Prolidases, also known as Xaa-Pro dipeptidases, are metalloproteases that catalyze the hydrolysis of dipeptides containing a C-terminal proline residue. Prolidases share a number of conserved sequence and structural features. These enzymes possess an N-terminal domain and a C-terminal catalytic domain, and form dimers through contact between both domains in a head-to-tail arrangement. The catalytic site features a binuclear metal cluster in the center of a pita-bread fold that is a canonical feature of this family of enzymes. Here we report the structure of E. coli PepQ, showing it to have the predicted pita-bread fold.

To better understand the potential significance of sequence conservation between the E. coli and human prolidases, we solved the structure of the bacterial enzyme at 2.0 Å resolution. The asymmetric unit contains a single PepQ dimer, which is the native oligomeric structure of this protein, arranged head-to-tail with inter-dimer contacts made between both domains. The active site of E. coli PepQ also features canonical metal binding residues, Asp246, Asp257, His339, Glu384 and Glu423, chelating two metal ions. Because PepQ was crystallized in buffer containing magnesium, the density found in this region is most likely derived from magnesium ions. Additionally, the mF0-DFc difference map shows greater density for one of the two metal ions (chelated by His339), consistent with reports from other pita-bread fold peptidases that this binding site has a higher affinity for metal ions. The decreased occupancy at the second metal site is surprising, given that the magnesium concentration during crystallization was in the millimolar range. This observation suggests that the affinity for magnesium of either PepQ in general, or this site in particular, is not as high as seen for the preferred manganese ion in related proteins, reported to be in the low- or sub-micromolar range [22], [34], [41]. Asp45, which reaches into the active site of one monomer from a loop region in the N-terminal domain of the other monomer, is seen in E. coli to be within interaction distance of Arg370, with the charged ends of the side chains approximately 3.5Å apart. PepQ Arg370, which is projected further into the active site on one of the loop regions conserved in prolidases from higher organisms, is placed far enough into the active site that it would physically impede the binding of longer peptides, as seen in the overlap between this arginine and the PepP-bound substrate tripeptide. PepQ R370 is, however, in an appropriate position for the guanidinium group of the arginine to interact with the C-terminus of the proline residue.

>[2x]MESLASLYKNHIATLQERTRDALARFKLDALLIHSGELFNVFLDDHPYPFKVNPQFKAWVPVTQVPNCWLLVDGVNKPKLWFYLPVDYWHNVEPLPTSFWTEDVEVIALPKADGIGSLLPAARGNIGYIGPVPERALQLGIEASNINPKGVIDYLHYYRSFKTEYELACMREAQKMAVNGHRAAEEAFRSGMSEFDINIAYLTATGHRDTDVPYSNIVALNEHAAVLHYTKLDHQAPEEMRSFLLDAGAEYNGYAADLTRTWSAKSDNDYAQLVKDVNDEQLALIATMKAGVSYVDYHIQFHQRIAKLLRKHQIITDMSEEAMVENDLTGPFMPHGIGHPLGLQVHDVAGFMQDDSGTHLAAPAKYPYLRCTRILQPGMVLTIEPGIYFIESLLAPWREGQFSKHFNWQKIEALKPFGGIRIEDNVVIHENNVENMTRDLKLA>[2x]MVIASVEDGGDGDTSKDDWLWYKQPASQTDATATAGGNYGNPDNNRWQQTTLPFGNGKIGGTVWGEVSRERVTFNEETLWTGGPGSSTSYNGGNNETKGQNGATLRALNKQLANGAETVNPGNLTGGENAAEQGNYLNWGDIYLDYGFNDTTVTEYRRDLNLSKGKADVTFKHDGVTYTREYFASNPDNVMVARLTASKAGKLNFNVSMPTNTNYSKTGETTTVKGDTLTVKGALGNNGLLYNS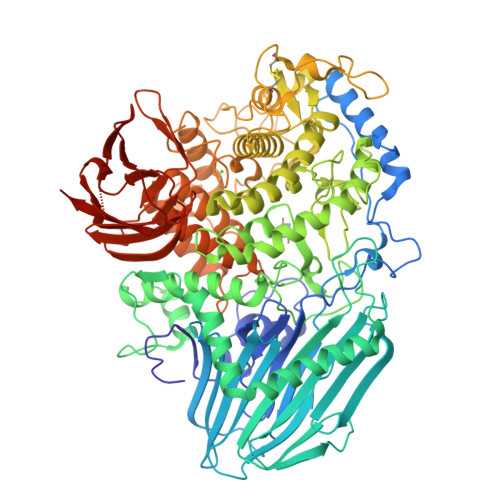QIKVVLDNGEGTLSEGSDGASLKVSDAKAVTLYIAAATDYKQKYPSYRTGETAAEVNTRVAKVVQDAANKGYTAVKKAHIDDHSAIYDRVKIDLGQSGHSSDGAVATDALLKAYQRGSATTAQKRELETLVYKYGRYLTIGSSRENSQLPSNLQGIWSVTAGDNAHGNTPWGSDFHMNVNLQMNYWPTYSANMGELAEPLIEYVEGLVKPGRVTAKVYAGAETTNPETTPIGEGEGYMAHTENTAYGWTAPGQSFSWGWSPAAVPWILQNVYEAYEYSGDPALLDRVYALLKEESHFYVNYMLHKAGSSSGDRLTTGVAYSPEQGPLGTDGNTYESSLVWQMLNDAIEAAKAKGDPDGLVGNTTDCSADNWAKNDSGNFTDANANRSWSCAKSLLKPIEVGDSGQIKEWYFEGALGKKKDGSTISGYQADNQHRHMSHLLGLFPGDLITIDNSEYMDAAKTSLRYRCFKGNVLQSNTGWAIGQRINSWARTGDGNTTYQLVELQLKNAMYANLFDYHAPFQIDGNFGNTSGVDEMLLQSNSTFTDTAGKKYVNYTNILPALPDAWAGGSVSGLVARGNFTVGTTWKNGKATEVRLTSNKGKQAAVKITAGGAQNYEVKNGDTAVNAKVVTNADGASLLVFDTTAGTTYTITKKAS VP24, one of only eight proteins encoded by ebolaviruses, functions in virus replication and assembly, and is thought to contribute to immune suppression by binding to a certain class of molecules called karyopherins to prevent them from transporting a transcription factor termed STAT1. In addition to its role in interferon antagonism, ebolavirus VP24 has also been proposed to associate with membranes, and is important for assembly and function of the viral ribonucleoprotein complex (RNP), where VP24 binds to the viral nucleoprotein NP. VP24 adopts a compact, single domain, α/β structure of novel fold (DaliLite v.3). The overall shape of VP24 resembles a triangular pyramid of dimensions 73 Å×30 Å×30 Å.

In order to provide 3D templates for understanding VP24 and its many roles in immune evasion, replication and assembly, we crystallized VP24 from Sudan virus (two versions crystallized: SUDV1–233 and SUDV11–233) and Reston virus (one version crystallized: RESTV11–237). We subsequently determined structures of SUDV1–233 and RESTV11–237 by molecular replacement, both at 2.0 Å resolution. The exception is RESTV, which appears to be non-pathogenic in humans, although it remains pathogenic to non-human primates. However, microarray analyses have shown that RESTV has a reduced ability to suppress host immune responses. Crystal structures presented here include VP24 from an ebolavirus that is pathogenic to humans (Sudan virus; SUDV) and VP24 from an ebolavirus that thus far, appears nonpathogenic to humans (Reston virus; RESTV), although it is lethal to nonhuman primates. The overall folds of SUDV and RESTV VP24 are similar, as expected (r.m.s.d. of 0.81 Å; also see Figure S2b for structural alignment). The entrance to the hydrophobic cavity (11 Å wide) appears to be gated by two residues (Y172 and M71) that point away from each other in RESTV VP24 but toward each other in SUDV VP24, appearing to block the hydrophobic cavity. Mapping of sequence differences between RESTV and the major pathogenic ebolaviruses (SUDV and EBOV) onto the RESTV11–237 structure indicates that RESTV VP24 differs in ∼30 sites. One of these sites, a cluster of residues L136, R139 and S140 (in RESTV), is next to the 142–146 loop, which is important for binding karyopherin α1 (Figure S4 and Figure S2a for sequence alignment). A second site is the cluster of residues L107, H109, T116 and G120 that exists within the 106–121 polypeptide that exhibits decreased H/D exchange in complex with STAT11–683 and may serve as a STAT1 binding site. Residues in VP24 that are unique to RESTV often colocalize with residues that appear to be important for karyopherin and STAT1 binding, or are important for virulence in rodents through an unknown mechanism.

>MAHHHHHHVDDDDKMVPPKKDMEKGVIFSDLCNFLITQTLQGWKVYWAGIEFDVSQKGMALLTRLKTNDFAPAWAMTRNLFPHLFQNPNSVIQSPIWALRVILAAGLQDQLLDHSLVEPLTGALGLISDWLLTTTSTHFNLRTRSVKDQLSLRMLSLIRSNILQFINKLDALHVVNYNGLLSSIEIGTSTHTIIITRTNMGFLVEVQEPDKSAMNSKRPGPVKFSLLHESAFKPFT[2x]>[2x]MNTFHVDFAPNTGEIFAGKQPGDVTMFTL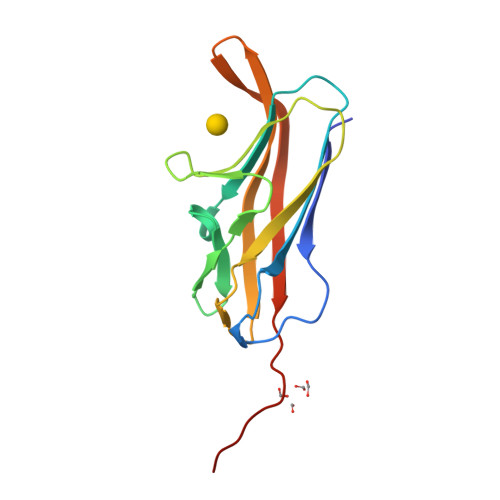TMGDTAPHGGWRLIPTGDSKGGYMISADGDYVGLYSYMMSWVGIDNNWYINDDSPKDIKDHLYVKAGTVLKPTTYKFTGRVEEYVFDNKQSTVINSKDVSGEVTVKQGLEHHHHHH> GSHMEFGIDLEFDADVQTMSPEASEYETCYVTSHKGPCRVATYSRDGQLIATGSADASIKILDTERMLAKSAMPIEVMMNETAQQNMENHPVIRTLYDHVDEVTCLAFHPTEQILASG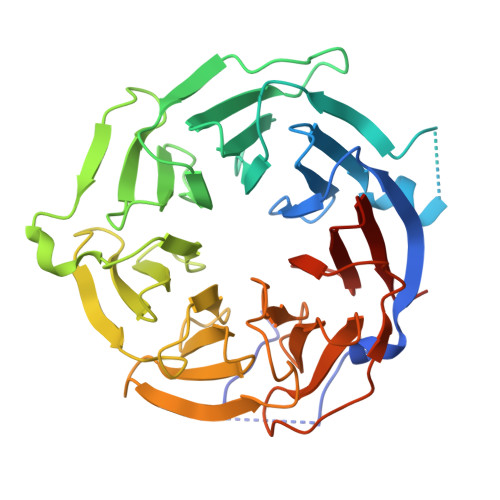SRDYTLKLFDYSKPSAKRAFKYIQEAEMLRSISFHPSGDFILVGTQHPTLRLYDINTFQCFVSCNPQDQHTDAICSVNYNSSANMYVTGSKDGCIKLWDGVSNRCITTFEKAHDGAEVCSAIFSKNSKYILSSGKDSVAKLWEISTGRTLVRYTGAGLSGRQVHRTQAVFNHTEDYVLLPDERTISLCCWDSRTAERRNLLSLGHNNIVRCIVHSPTNPGFMTCSDDFRARFWYRRSTTD> AQIGPVTDLHITNANISPDGFSRPAVLAGGTFPGPTIAGNTGDNFQITVFNDLTDPSMLTDTSIHWHGLFQKGTNWADGPAFVTQCPIITGQSFDYNFNVPGQAGTFWYHSHLSTQYCDGLRGPFVVYDPNDPNASLYDVDDDTTIITLADWYHTLAQQEPIGAAITADATLINGLGRSFTNTTASPLSVITVQSGK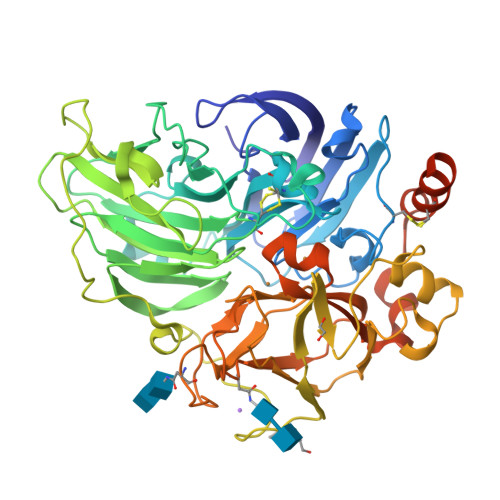RYRMRLVSISCDPNYLFSIDGHDMTIIEVDGVNSQQLTVDQIQIFAAQRYSFVLNANQPVGNYWIRAQPNSGGQGFDGGINSAILRYEGATVEDPTTTAPTTFSNPLVETDLHPLADLGVPGQPFRGGADDPLVLNLAFANGRFSIDGVSFVPPTVPVLLQILSGAQNAQDLLPAGSVISLPSNSVIEVALPAGAAGGPHPFHLHGHNFAVVQSANNATPNYVNPIWRDTVSIGGTGDNVTIRFTTNNPGPWFLHCHIDWHLEAGFAIVFAEDIPDTASANPVPQAWSDLCPAYDQAHNISTATRQDFQILCICGILHVNFRQEERCGIS2-chloranyl-4-[2-(3-chloranyl-4-oxidanyl-phenyl)propan-2-yl]phenol | C15 H14 Cl2 O2 | 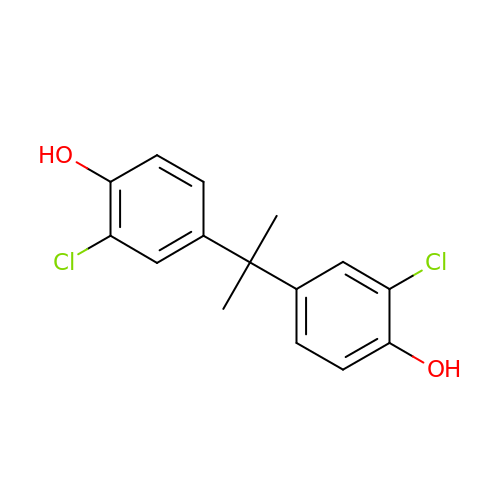XBQRPFBBTWXIFI-UHFFFAOYSA-N>[2x]MENKIEVNSKDEMNKWFEEFKKGNGLVDTYTNSYSFCESVPNLDRFVFQMAGA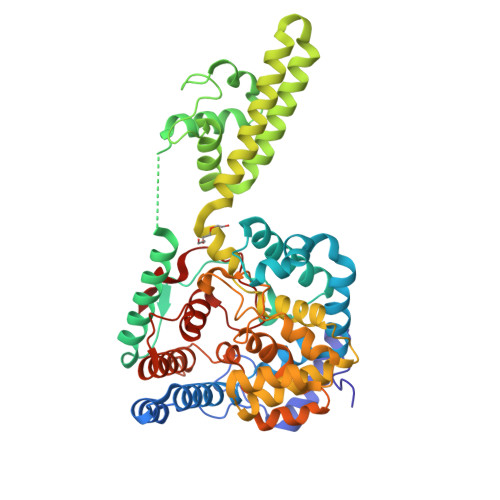TDDAQKDSIYASALVEATKFCAPIYECAWASSTGIVKKGLEWFEKNTGTIKSWDESYIELKVEVPKIEQLFNYQQAALKWRKDIGFRVNANTAALSNKVLAEYKVPGEIVMSVKEMLSDMIRRRNLILNRGGDENPRGPVSHEHVEWCREFVKGKYIMAFNPPWGDINKSGRSGIALVATGLAKLAETEGKGVFDEAKKTVEALNGYLDKHKDEVDKASADNMVTNLLKHVAKAQELYKNSSALRAQGAQIDTVFSSYYWLYKAGVTPETFPTVSQFLFELGKHPRGTKKMKKALLSTPMKWGKKLYELFADDSFQQNRIYMHPAVLTAGRISEMGVCFGTIPVANPDDAALGSGHTKSILNLRTNTETNNPCARTIVKLFEIQKTGFNIQDMDIVASEHLLHQSLVGKQSPFQNAYNVKGNATSANII> MGMLEARELLCERDERTLFSGLSFTLNAGEWVQITGSNGAGKTTLLRLLTGLSRPDAGEVLWQGQPLHQVRDSYHQNLLWIGHQPGIKTRLTALENLHFYHRDGDTAQCLEALAQAGLAGFEDIPVNQLSAGQQRRVALARLWLTRATLWILDEPFTAIDVNGVDRLTQRMAQHTEQGGIVILTTHQP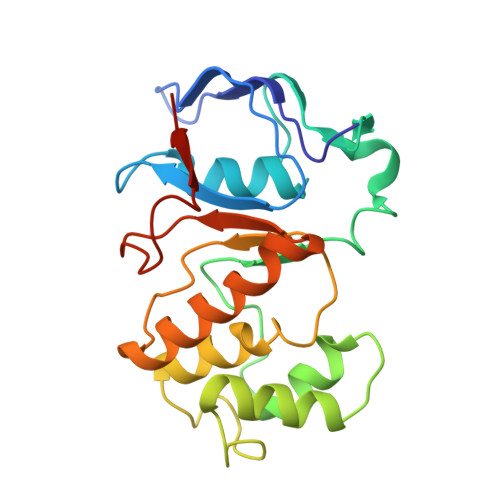LNVAESKIRRISLTQTRAA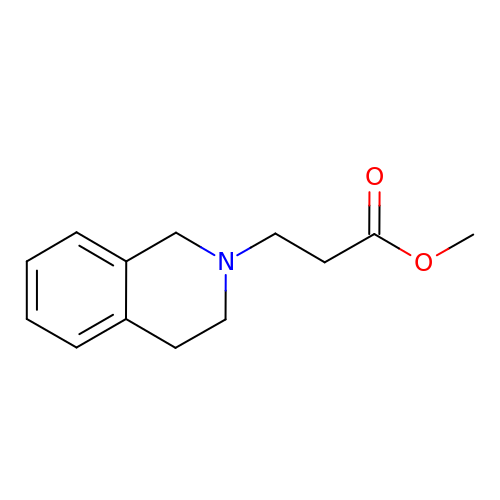methyl 3-(3,4-dihydroisoquinolin-2(1H)-yl)propanoate | C13 H17 N O2 | LGCHTHNCFDGWBW-UHFFFAOYSA-N> MGHHHHHHHHHHSSGHIEGRHMFSKNAVKLHATPPSVAAPPTGAPEVAAERLEPRVEEKDGYWILKEQFRKGINPQEKVKIEKEPMKLFMENGIEELAKIPIEEIDQSKLTKDDIDVRLKWLGLFHRRKNQYGRFMMRLKLPNGVTTSAQTRYLASVIRKYGKEGC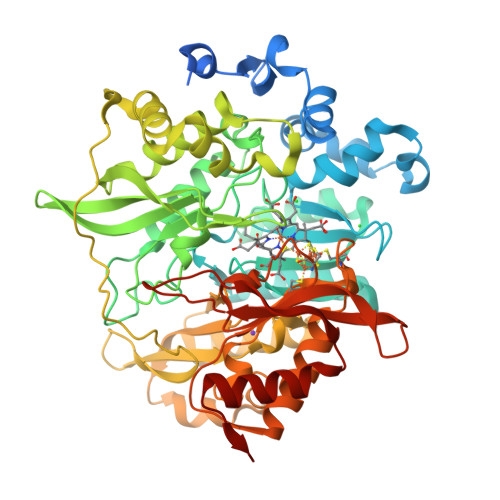ADITTRQNWQIRGVVLPDVPEILKGLAEVGLTSLQSGKDNVRNPVGNPLAGIDPEEIVDTRPYTNLLSQFITGNSRGNPAVSNLPRKWNPCVVGSHDLYEHPHINDLAYMPATKDGRFGFNLLVGGFFSAKRCDEAIPLDAWVPADDVVPVCRAILEAFRDLGFRGNRQKCRMMWLIDELGVEGFRAEVEKRMPQQQLERASPEDLVQKQWERRDYLGVHPQKQEGYSFIGLHIPVGRVQADDMDELARLADEYGSGEIRLTVEQNIIIPNIETSKIEALLKEPVLSTFSPDPPILMKGLVACTGNQFCGQAIIETKARSLKITEEVQRQVSLTKPVRMHWTGCPNTCAQVQVADIGFMGCLTRDKNGKTVEGADVFLGGRIGSDSHLGEVYKKAVPCDDLVPLVVDLLVNNFGAVPR>MRYKKKWAATEPKFPAVRLALQNFDMTYSVQFGDLWPSIRVSLLSEQKYGALVNNFAAWDHVSAKLEQLSAKDFVNEAISHWELQSEGGQSAAPSPASWACSPNLRCFTFDRGDISRFPPARPGSLGVMEYYLMDAASLLPVLALGLQPGDIVLDLCAAPGGKTLALLQTGCCRNLAANDLSPSRIARLQKILHSYVPEEIRDGNQVRVTSWDGRKWGELEGDTYDRVLVDVPCTTDRHSLHEEENNIFKRSRKKERQILPVLQVQLLAAGLLATKPGGHVVYSTCSLSHLQNEYVVQGAIELLANQYSIQVQVEDLTHFRRVFMDTFCFFSSCQVGELVIPNLMANFGPMYFCKMRRLT[4x];>[4x]SNGGVIEELSCVRSNNYVQEPECRRNLVQCLLEKQGTPVVQGSLELERVMSSLLDMGFSNAHINELLSVRRGASLQQLLDIISEFILLGLNPEPVCVVLKKSPQLLKLPIMQMRKRSSYLQKLGLGEGKLKRVLYCCPEIFTMRQQDINDTVRLLKEKCLFTVQQVTKILHSCPSVLREDLGQLEYKFQYAYFRMGIKHPDIVKSEYLQYSLTKIKQRHIYLERLGRYQTPDKKGQTQIPNPLLKDILRVSEAEFLARTACTSVEEFQVFKKLLAREEEES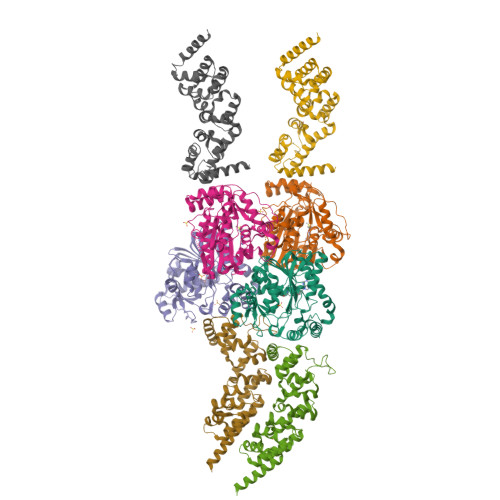ESSTSDDKRASLDEDEDDDDEEDNDEDDNDEDDDDEDDDEAEDNDEDEDDDEEE> GPLGSPLTASMLASAPPQEQKQMLGERLFPLIQAMHPTLAGKITGMLLEIDNSELLHMLESP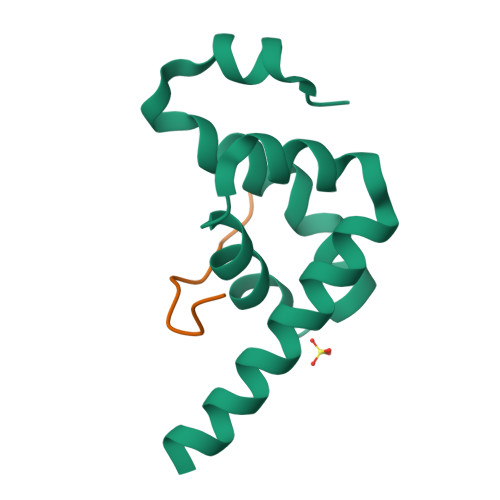ESLRSKVDEAVAVLQAHQAKEAAQKA;> TGLNPNAKVWQEIA> MEYEWKPDEQGLQQILQLLKESQSPDTTIQRTVQQKLEQLNQYPDFNNYLIFVLTKLKSEDEPTRSLSGLILKNNVKAHFQNFPNGVTDFIKSECLNNIGDSSPLIRATVGILITTIASKGELQNWPDLLPKLCSLLDSEDYNTCEGAFGALQKICEDSAEILDSDVLDRPLNIMIPKFLQFFKHSSPKIRSHAVACVNQFIISRTQALMLHIDSFIENLFALAGDEEPEVRKNVCRALVMLLEVRMDRLLPHMHNIVEYMLQRTQDQDENVALEACEFWLTLAEQPICKDVLVRHLPKLIPVLVNGMKYSDIDIILLKGDVEEDETIPDSEQDIRPRFHRSRTVAQQHDEDGIEEEDDDDDEIDDDDTISDWNLRKCSAAALDVLANVYRDELLPHILPLLKELLFHHEWVVKESGILVLGAIAEGCMQGMIPYLPELIPHLIQCLSDKKALVRSITCWTLSRYAHWVVSQPPDTYLKPLMTELLKRILDSNKRVQEAACSAFATLEEEACTELVPYLAYILDTLVFAFSKYQHKNLLILYDAIGTLADSVGHHLNKPEYIQMLMPPLIQKWNMLKDEDKDLFPLLECLSSVATALQSGFLPYCEPVYQRCVNLVQKTLAQAMLNNAQPDQYEAPDKDFMIVALDLLSGLAEGLGG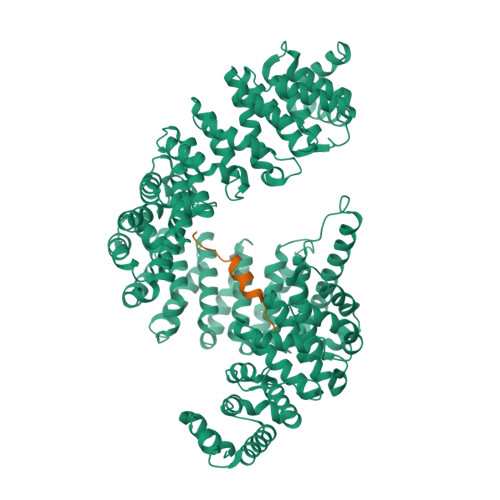NIEQLVARSNILTLMYQCMQDKMPEVRQSSFALLGDLTKACFQHVKPCIADFMPILGTNLNPEFISVCNNATWAIGEISIQMGIEMQPYIPMVLHQLVEIINRPNTPKTLLENTAITIGRLGYVCPQEVAPMLQQFIRPWCTSLRNIRDNEEKDSAFRGICTMISVNPSGVIQDFIFFCDAVASWINPKDDLRDMFCKILHGFKNQVGDENWRRFSDQFPLPLKERLAAFYGV;> GPLGSRGGRGGGDRGGFGPGKMDSRGEHRQDRRERPY>[2x]MAHHHHHHMNTDERYKLLRSVGEECIQESELRNLIEKKPLIRCYDGFEPSGRMHIAQGIFKAVNVNKCTAAGCEFVFWVADWFALMNDKVGGELEKIRIVGRYLIEVWKAAGMDMDKVLFLWSSEEITSHADTYWRMVLDIGRQNTIARIKKCCTIMGKTEGTLTAAQVLYPLMQCCDIF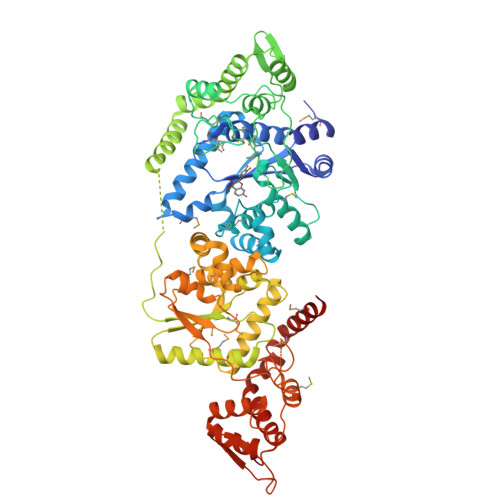FLKADICQLGLDQRKVNMLAREYCDLIGRKLKPVILSHHMLAGLKQGQAKMSKSDPDSAIFMEDTEEDVARKIRQAYCPRVKQSASAITDDGAPVATDDRNPVLDYFQCVVYARPGAAATIDGTTYATYEDLEQAFVSDEVSEDALKSCLIDEVNALLEPVRQHFASNEEAHELLEAVKSYRKDGATLPLAETALPAAPAKPHACMWMPALLKVPLDVAEGMIKVTKDFIAAHPEGTVTLVLPDWSAVASDEITGVEKDISAALQVNCALLKAYGLPSSVKIVTENEVILGNCDDFWVSVIGIARKNLLSHVEELYGGEVRNAGQVIAALMRVATALMLSVSHVISTSLDGHINAFAREYTKERIDCVQTLEGRIPALHRPGAAPAVLGADDVLYLDDNDMDIRRKIKKAYSAPNEEANPVISVAQHLLAQHGALSIERGEANGGNVSYNTPEALVADCGSGALHPADLKAAVLQLLLDRSAQARALLNGELKKNMTVLRNAEKKMAKKR>DVPLTPSQFAKAKSENFDKKVILSNLNKPHALLWGPDNQIWLTERATGKILRVNPESGSVKTVFQVPEIVNDADGQNGLLGFAFHPDFKNNPYIYISGTFKNPKSTDKELPNQTIIRRYTYNKSTDTLEKPVDLLAGLPSSKDHQSGRLVIGPDQKIYYTIGDQGRNQLAYLFLPNQAQHTPTQQELNGKDYHTYMGKVLRLNLDGSIPKDNPSFNGVVSHIYTLGHRNPQGLAFTPNGKLLQSEQGPNSDDEINLIVKGGNYGWPNVAGYKDDSGYAYANYSAAANKSIKDLAQNGVKVAAGVPVTKESEWTGKNFVPPLKTLYTVQDTYNYNDPTCGEMTYICWPTVAPSSAYVYKGGKKAITGWENTLLVPSLKRGVI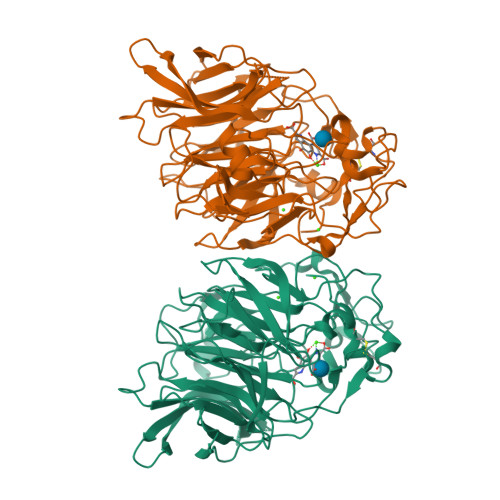FRIKLDPTYSTTYDDAVPMFKSNNRYRDVIASPDGNVLYVLTDTAGNVQKDDGSVTNTLENPGSLIKFTYKAK[2x]> GGCUUAUCAAGAGAGGUGAAGGGACUGGCCCGACGAAACCCGGCAACCAGAAAUGGU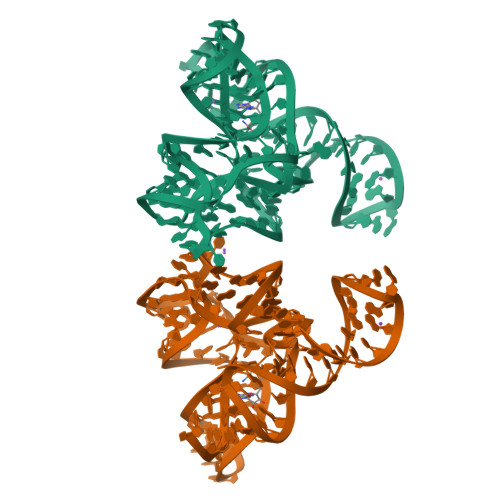GCCAAUUCCUGCAGCGGAAACGUUGAAAGAUGAGCCGA>GSHMVAAGDNKIKQGLLPSLEDLLFYTIAEGQEKIPVHKFITALKSTGLRTSDPRLKECMDMLRLTLQTTSDGVMLDKDLFKKCVQSNIVLLTQAFRRKFVIPDFMSFTSHIDELYESAKKQSGGKVADYIPQLAKFSPDLWGVSVCTVDGQRHSIGDTKVPFCLQSCVKPLKYAIAVNDLGTEYVHRYVGKEPSGLRFNKLFLNEDDKPHNPMVNAGAIVVTSLIKQGVNNAEKFDYVMQFLNKMAGNEYVGFSNATFQSERESGDRNFAIGYYLKEKKCFPEGTDMVGILDFYFQLCSIEVTCESASVMAATLANGGFCPITGERVLSPEAVRNTLSLMHSCGMYDFSGQ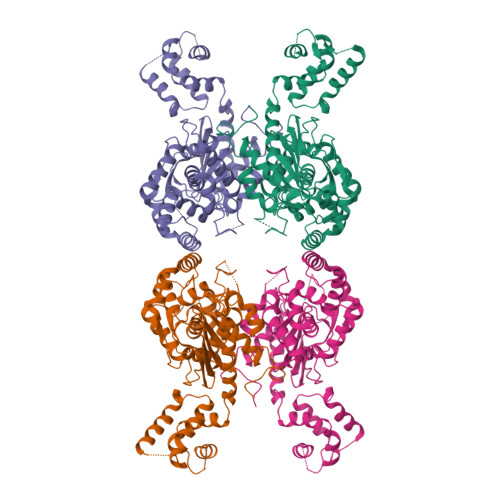FAFHVGLPAKSGVAGGILLVVPNVMGMMCWSPPLDKMGNSVKGIHFCHDLVSLCNFHNYDNLRHFAKKLDPRREGGDQRHSFGPLDYESLQQELALKDTVWKKVSPESSDDTSTTVVYRMESLGERS[4x]>[2x]SSSYTEADPAI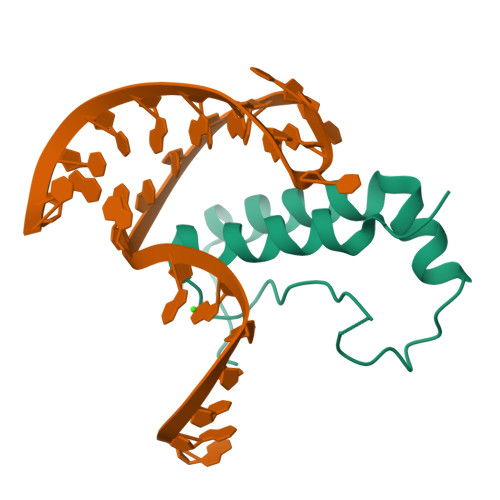LSRRQKQIDYGKNTAAYERYVEMVPKDERTRDHPRTPNKYGKYSRRAFDGLVKIWRKSLHIYDPPTQARDTAKDSNSDSDSD> MSPSMQQRTDLP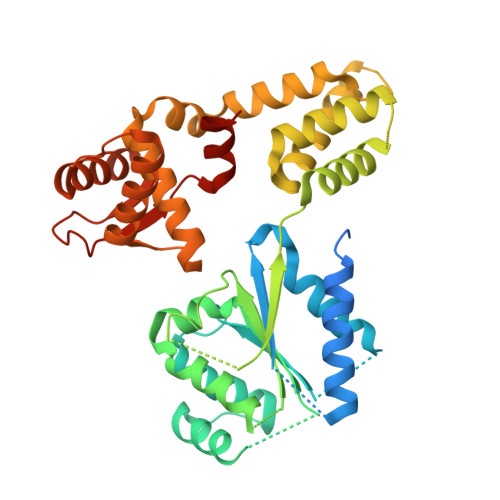AKDSSKSELQLAREQLHVSVVPKSLPCREREFENIYAFLEGKIQDQCGGCMYVSGVPGTGKTATVTGVIRTLQRMAKQNELPAFEYLEINGMRLTEPRQAYVQIYKQLTGKTVSWEQAHALLEKRFTTPAPRRVTTVLLVDELDILCNRRQDVVYNLLDWPTKSAAKLVVVTIANTMDLPERLLMGKVTSRLGLTRLTFQPYSHKQLQEIVTARLGGSETFKGEAVQLVARKVAAVSGDARRALDICRRATEIADTAAVKCVTMLHVQQALAEMIASAKVQAIRNCSRMEQIFLQAIAAEVTRTGVEETTFMGVYQQVETIAAFMGVTFPPPGRALRLCSKLGAERLIISEHSRNDLFQKILLNVSADDIHYALRVEEMVN> MSAPTDDTPTDAIAAPRHSAPPRPRLPWFLRTFAVPIILAWVAVVAILNTVVPTLDEVGEMRAVSMAPNDAPSTLAIKRVGQVFEEYDTSSSVMIVLEGEEPLGIEAHAFYDKMVADLRADTEHVQHVQDFWGDTLTASGAQSVDGKAAYVQVYIAGDQGESLANESVEAVRKIATERETPSGVKAYVTGAAATSADQRAEGDASMKLIEGVTFAVITVMLLAVYRSVITTLIVLAMVVLGLSGARGIVAFLGFYNVFGLTTFATNMVVTLAIAAATDYAIFLIGRYQEARRAGEDRESAYYTMFHGTAHVVLASGLTIAGATLCLHFTRLPYFQTMGVPLAIGMLIVVAAALTAGPAVISVVSRFGKTLEPKRFSRSPGWHRVGTATVRWPGAILVCAVVAALIGLLALPGYYTTYDDRRYLPDDVPANVGYDAAFRHFSQAKMNPDLMMVETDRDLRNPADFLVIDKIAKALKNVHGIAQVQTITRPDGDPIEHSTIPYTIGQSGTTQIMNNDYMQTNLDNLLKQADDLQTSIDSMTEMMNIQTELAAVSQSMADKMAQTSDDTADVRDHLADFDDFFRPIRNYLYWEPHCYDIPMCWSMRSIFESIDGINTMSDDFQELVPEMRRMADLMPRMVAVMPAQIQSMKNQKQTLLNQYQVQKAQQDQNMAMQENATAMSQAFDAAKNDDSFYLPPEAFETDDFQRGMKLFMSPDGHAVRFTIIHQGDPLTEEGTARMDELKVAAADAIKGTPFEGARIYLGGSAATYNDMQIGADYDLIIVAASALILIFIIMMVLTRAVVAAAVIVGTVVLSLASAFGLSVLLWQHIVGIPLHWMVLPMSVIVLLAVGADYNLLLVSRMKEEIHAGIRTGIIRAMV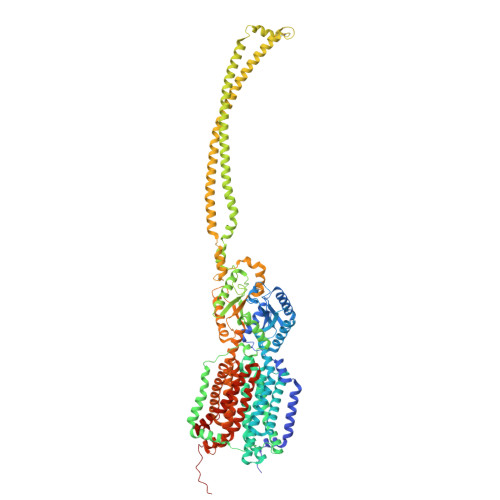GTGAVVTAAGLVFAFTMASMAVSSLITIGQVGTTIGLGLLFDTLVVRSLMTPSIATLLGRWFWWPQRVRERPVPSKWPTPIQRTPEEALS>MNLKDKILGVAKELFIKNGYNATTTGEIVKLSESSKGNLYYHFKTKENLFLEILNIEESKWQEQWKKEQIKAKTNREKFYLYNELSLTTEYYYPLQNAIIEFYTEYYKTNSINEKMNKLQNKYIDAYHVIFKEGNLNGEWSINDVN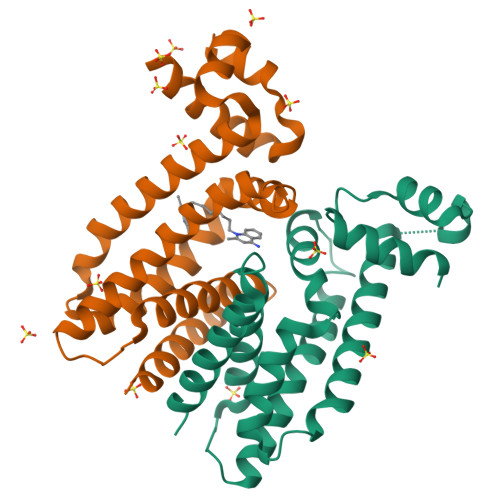AVSKIAANAVNGIVTFTHEQNINERIKLMNKFSQIFLNGLSKHHHHHH[4x]> AAPTAYTPLDVAQAYQFPEGLDGQGQCIAIIELGGGYDETSLAQYFASLGVSAPQVVSVSVDGATNQPTGDPNGPD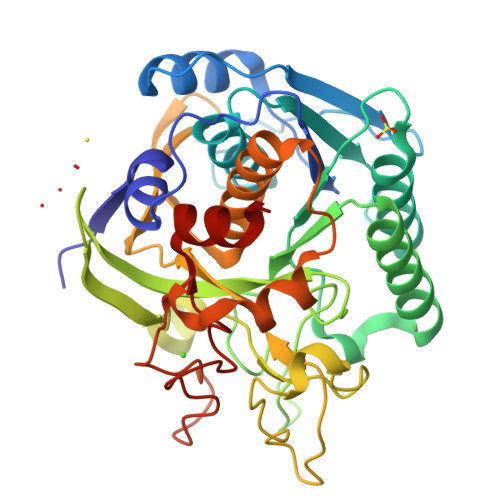GEVELDIEVAGALAPGAKIAVYFAPNTDAGFLNAITTAVHDPTHKPSIVSISAGGPEDSWAPASIAAMNRAFLDAAALGVTVLAAAGDSGSTDGEQDGLYHVDFPAASPYVLACGGTRLVASAGRIERETVWNDGPDGGSTGGGVSRIFPLPSWQERANVPPSANPGAGSGRGVPDVAGNADPATGYEVVIDGETTVIGGTSAVAPLFAALVARINQKLGKPVGYLNPTLYQLPPEVFHDITEGNNDIANRARIYQAGPGWDPCTGLGSPIGIRLLQALLPSASQAQP N-{3-[(4S,6R)-2-amino-4-methyl-6-(trifluoromethyl)-5,6-dihydro-4H-1,3-oxazin-4-yl]-4-fluorophenyl}-5-cyanopyridine-2-carboxamide | C19 H15 F4 N5 O2 | 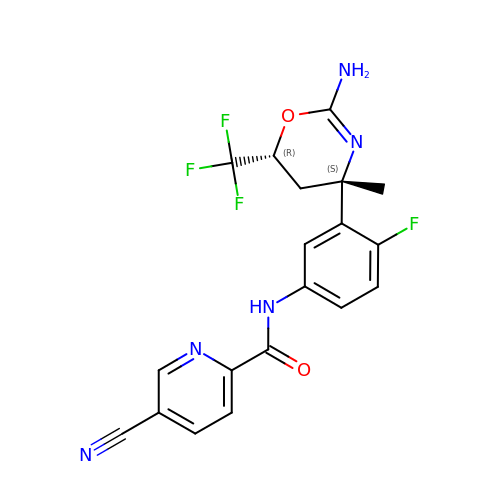MELQHVBGGSKVJQ-QAPCUYQASA-N>MSQSNRELVVDFLSY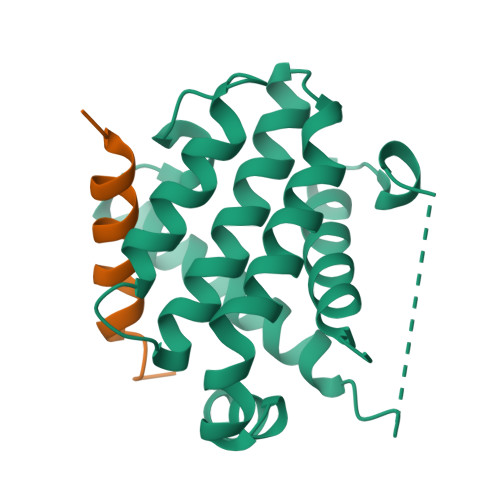KLSQKGYSWSQFSDVEENRTEAPEGTESEMAAVKQALREAGDEFELRYRRAFSDLTSQLHITPGTAYQSFEQVVNELFRDGVNWGRIVAFFSFGGALCVESVDKEMQVLVSRIAAWMATYLNDHLEPWIQENGGWDTFVELYGNNAAAESRKGQER[4x];>[4x]HQAEVQIARKLQCIADQFHRLHVQQ>MTKWVLHVDLDQFLASVELRRRPDLRGQPVIVGGSGDPSEPRKVVTCASYEAREFGVHAGMPLRAAARRCPDATFLPSDPAAYDEASEQVMGLLRDLGHPLEVWGWDEAYLGADLPDESDPVEVAERIRTVVAAETGLSCSVGISDNKQRAKVATGFAKPAGIYVLTEANWMTVMGDRPPDALWGVGPKTTKKLAAMGITTVADLAVTDPSVLTTAFGPSTGLWLLLLAKGGGDTEVSSEPWVPRSRSHVVTFPQDLTERREMDSAVRDLALQTLAEIVEQGRIVTRVAVTVRTSTFYTRTKIRKLPA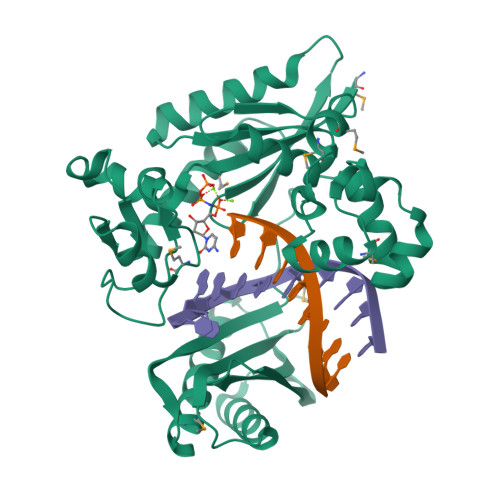PSTDAGQIVDTALAVLDQFELDRPVRLLGVRLELAMDDVPRPAVTAGT[2x]> MAQVKSSYSYDAPSDFINFSSLDDEGDTQNIDSWFEEKANL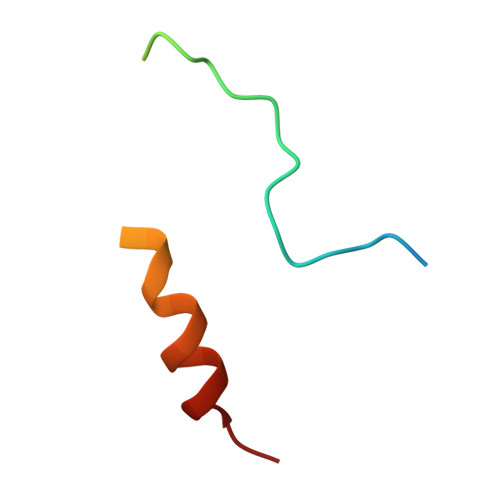EN> FAKEIDASCIKIEKVIGVGEFGEVCSGRLKVPGKREICVAIKTLKAGYTDKQRRDFLSEASIMGQFDHPNIIHLEGVVTKCKPVMIITEYMENGSLDAFLRKNDGRFTVIQLVGMLRGIGSGMKYLSDMSYVHRDLAARNILVNSNLVCKVSDFGMSRVLEDDPEAAYTTRGGKIPIRWTAPEAIAYRKFTSASDVWSYGIVMWEVMSYGERPYWDMSNQDV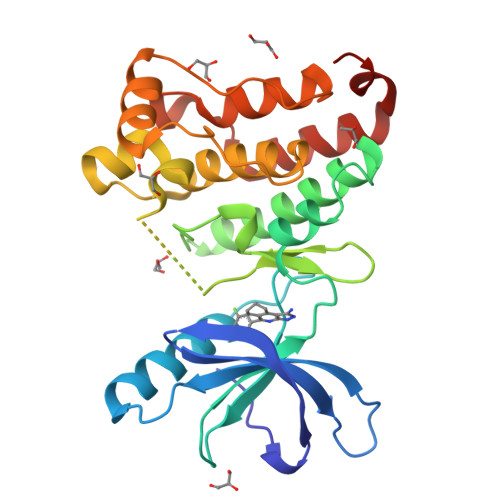IKAIEEGYRLPPPMDCPIALHQLMLDCWQKERSDRPKFGQIVNMLDKLIRNPNSLKRTGSESS>[2x]MARTFFVGGNFKLNGSKQSIKEIVERLNTASIPENVEVVICPPATYLDYSV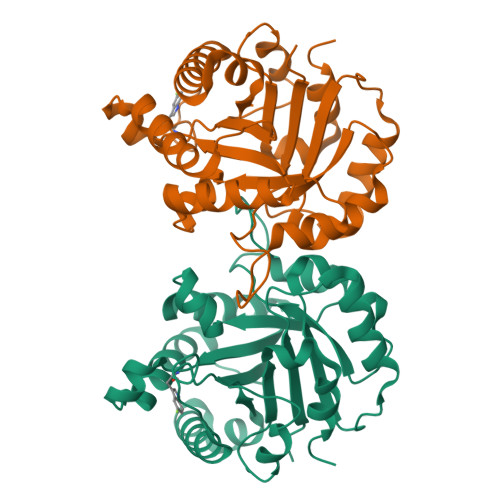SLVKKPQVTVGAQNAYLKASGAFTGENSVDQIKDVGAKYVILGHSERRSYFHEDDKFIADKTKFALGQGVGVILCIGETLEEKKAGKTLDVVERQLNAVLEEVKDFTNVVVAYEPVWAIGTGLAATPEDAQDIHASIRKFLASKLGDKAASELRILYGGSANGSNAVTFKDKADVDGFLVGGASLKPEFVDIINSRN>MGSSHHHHHHSSGRENLYFQGMKETNSEEADSGLAFFRNMYDKYRDAFLSHLNEYSLEEEIKEHISKYYKLLFDYNCLGGKNNRGILVILIYEYVKNRDINSSEWEKAACLAWCIEILQAAFLVADDIMDKGEMRRNKYCWYLLKDVETKNAVNDVLLLYNSIYKLIEIYLRNESCYVDVIATFRDATLKTIIGQHLDTNIFSDKYSDAHREIDVNNINVPEQPVIDINMINFGVYKNIVIHKTAYYSFFLPIVCGMLLAGIAVDNLIYKKIEDI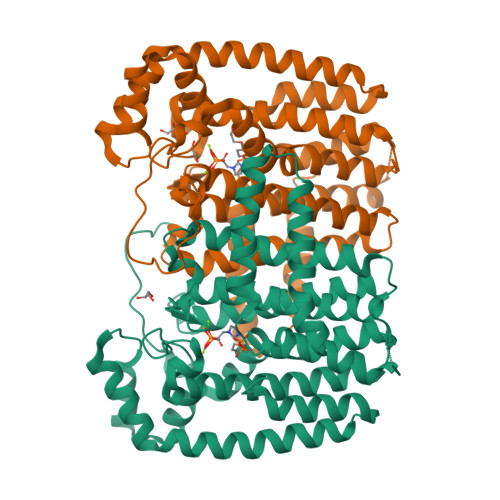SMLMGEYFQIHDDYLDIFGDSTKTGKVGSDIQNNKLTWPLIKTFELCSEPDKIKIVKNYGKNNLACVKVIDSLYEQYKIRKHYESYEKAQKAKILSAINELHHEGIEYVLKYLLEILFTGV[4x]> 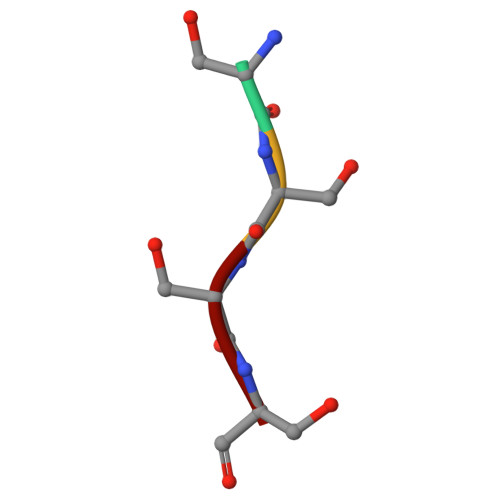SSSS>[2x]GPMNQLDQLGTRINLICNVFDKWIGQQDLNYNLFAVLYTLATEGSRTQKHIGEKWSLPKQTVSGVCKTLAGQGLIEWQEGEQDRRKRLLS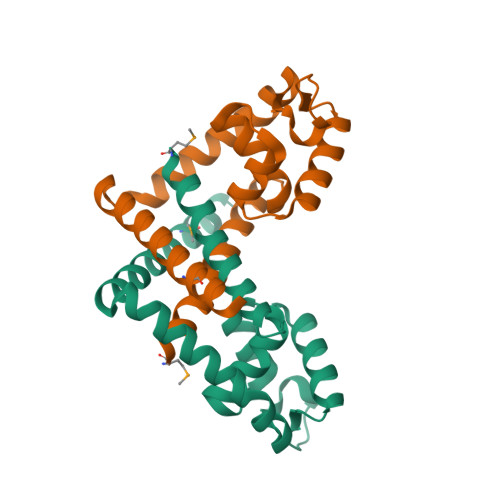LTETGKAYAAPLTESAQEFSDKVFATFGDKRTTRLFADLDALAEVMEKTISENKK>[2x]AVQQNKELNFKLREKQNEIFELKKIAETLRSKLEKY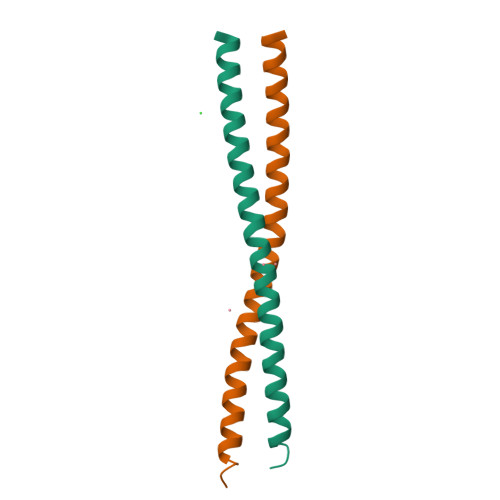VDITKKLEDQNLNLQIKISDLEKKLSDANSTFKEMRFP> MLELLPTAVEGVSQAQITGRPEWIWLALGTALMGLGTLYFLVKGMGVSDPDAKKFYAITTLVPAIAFTMYLSMLLGYGLTMVPFGGEQNPIYWARYADWLFTTPLLLLDLALLVDADQGTILALVGADGIMIGTGLVGALTKVYSYRFVWWAISTAAMLYILYVLFFGFTSKAESMRPE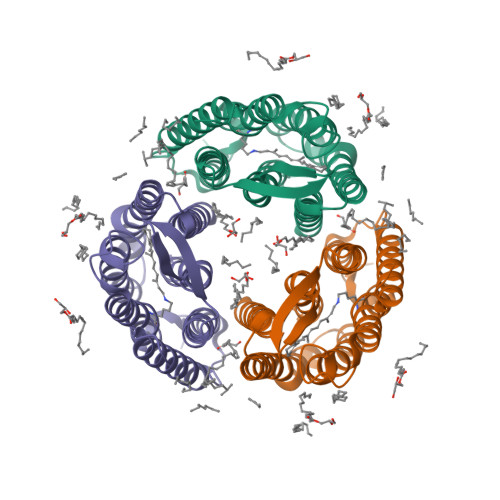VASTFKVLRNVTVVLWSAYPVVWLIGSEGAGIVPLNIETLLFMVLDVSAKVGFGLILLRSRAIFGEAEAPEPSAGDGAAATSD> DLYRHSSQYRMWSYTKDQLQEKRVDTNARAIAYIEENLLKFREAHNLTEEEIKVLEAKAIPLTMEEELDLVNFYAKKVQVIAQHLNLPTEVVATAISFFRRFFLENSVMQIDPKSIVHTTIFLACKSENYFISVDSFAQKAKSTRDSVLKFEFKLLESLKFSLLNHHPYKPLHGFFLDIQNVLYGKVDLNYMGQIYDRCKKRITAALLTDVVYFYTPPQITLATLLIEDEALVT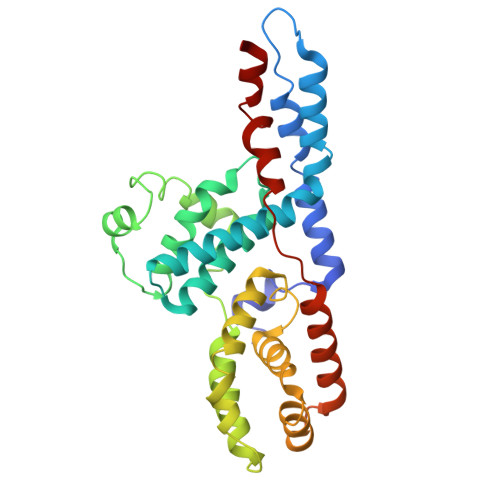RYLETKFPSREGSQESVPGNEKEEPQNDASTTEKNKEKSTESEEYSIDSAKLLTIIRECKSIIEDCKPPSTEEAKKIAAKNYYCQNPSTL>[2x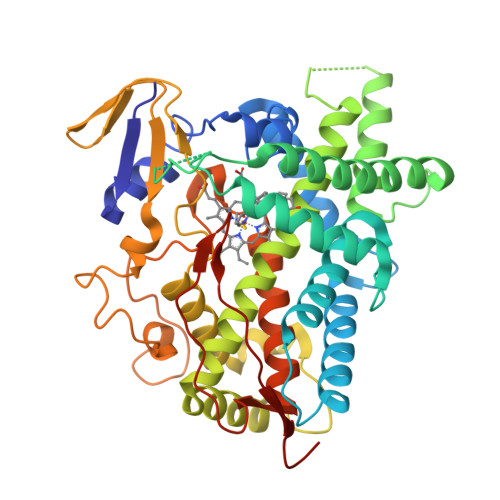]MGSHKLLIVNNHHHAKEILIKKGKIFAGRPRTVTTDLLTRDGKDIAFADYSSTWKFHRKMVHGALCMFGEGSVSIEKIICREASSMCEVLTESQNSAVDLGPELTRAVTNVVCALCFNSSYKRGDAEFESMLQYSQGIVDTVAKDSLVDIFPWLQIFPNKDLTILRQCISIRDKLLQKKYEEHKVTYSDNVQRDLLDALLRAKRSSENNNSSTRDVGLTEDHVLMTVGDIFGAGVETTTTVLKWSIAYLVHNPQVQRKIQEELDSKIGKERHPQLSDRGNLPYLEATIREVLRIRPVSPLLIPHVALQDSSVGEYTVQKGTRVVINLWSLHHDKKEWKNPELFDPGRFLNEEGDGLCCPSGSYLPFGAGVRVCLGEALAKMELFLFLAWILQRFTLEMPTGQPLPDLQGKFGVVLQPKKFKVVAKVRADWEKSPLMQHC> GPHMSIINYNEGQWSPNNPSGKKQYDREQLLQLREVKASRIQP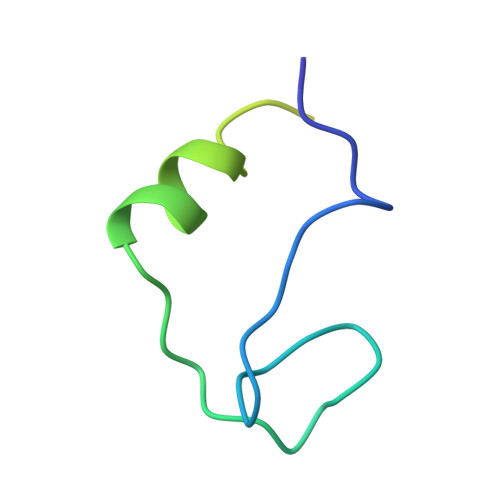EVKNVSILPQPNLMPSFIRNN> FCHPQN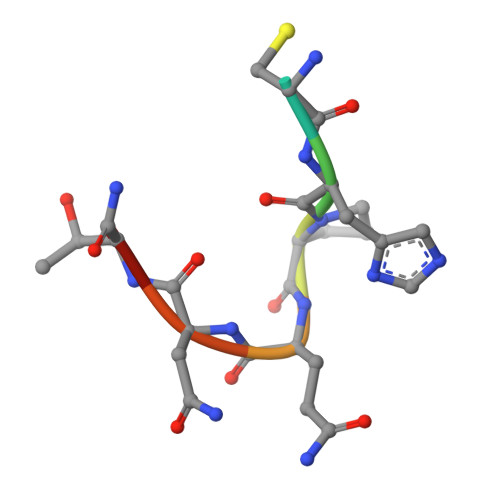TX> MRVLGIETSCDETGIAIYDDKKGLLANQLYSQVKLHADYGGVVPELASRDHVRKTVPL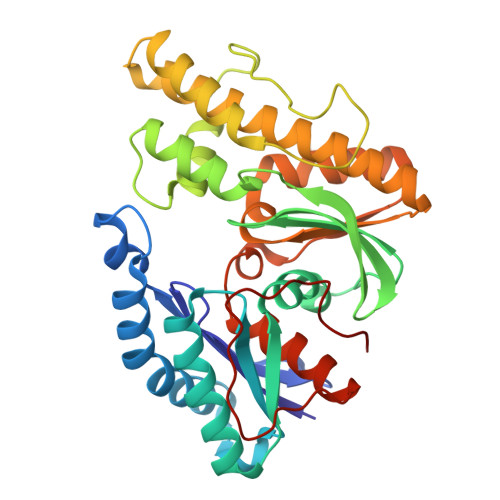IQAALKEAGLTASDIDAVAYTAGPGLVGALLVGATVGRSLAFAWNVPAIPVHHMEGHLLAPMLEDNPPEFPFVALLVSGGHTQLISVTGIGQYELLGESIDDAAGEAFDKTAKLLGLDYPGGPMLSKMASQGTAGRFVFPRPMTDRPGLDFSFSGLKTFAANTIRSNGGDEQTRADIARAFEDAVVDTLMIKCKRALESTGFKRLVMAGGVSANRTLRAKLAEMMQKRRGEVFYARPEFCTDNGAMIAYAGMVRFKAGVTADLGVTVRPRWPLAELPAA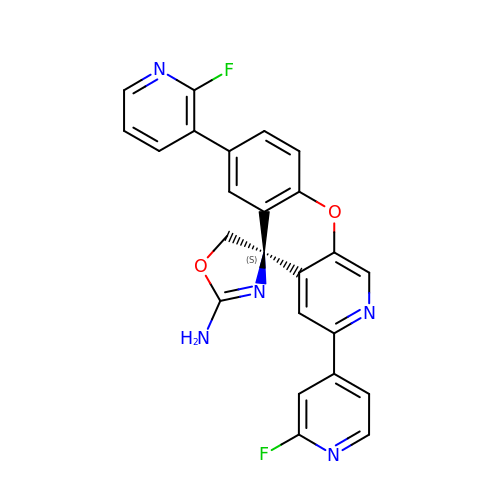(5S)-7-(2-fluoropyridin-3-yl)-3-(2-fluoropyridin-4-yl)spiro[chromeno[2,3-c]pyridine-5,4'-[1,3]oxazol]-2'-amine | C24 H15 F2 N5 O2 | LEFDLEYZSDTVMO-DEOSSOPVSA-N> MGHHHHHHHHHHSSGHIEGRHMGSGNGGTATAEGIPAKGTDDG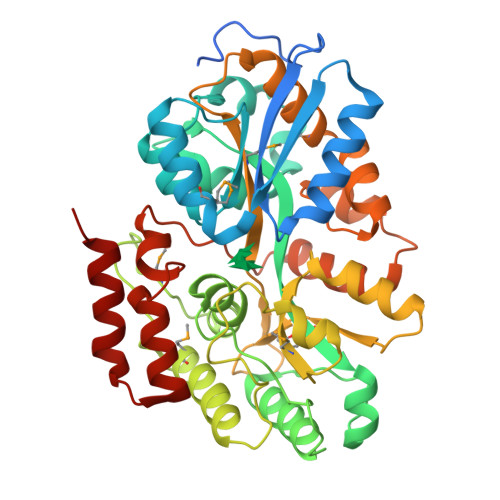TEITLWTRSPLERQAKNVVEAYNKSHKNQVKLEIIPNDDMEGKVGGASQTDSLPDILAGDVVRIPYWASEGIFTDITKQIDGLDNKADLQQGHIEAGTVDGAEYTLPFITDVSVMVWNKNLYKEAGLDPEQGPKSIDQFVEQAKKVAALNKDGVAGSYLAGQSGGALVFDLFPSVWADGESVMNKDGSEATLDNDSMKGVLDAYKELANTTNGLGAGSKEETGATWTAPFANGKIGVMPYPNTSTTALFDAEKDGGFEVGVAPIPGTKEGKTSTFLGGDAMGISKDSKHVAQAWNFLYWLMQSDAQKEVFADQGDTASNIQTLKTAYKDADPRIQTINSVIIDGNGQTPKSPAFNEAFNAAGSPWQLLVQNAVWGSGDLKADNKAVTDVLSAQ>MSLTTFLFRNGALLDPDHPDLLQGFEILIEDGFIREVSDKPIKSSNAHVIDVKGKTIMPGLIDLHVHVVAIEFNLPRVATLPNVLVTLRAVPIMRAMLRRGFTTVRDAGGAGYPFKQAVESGLVEGPRLFVSGRALSQTGGHADPRARSDYMPPDSPCGCCVRVGALGRVADGVDEVRRAVREELQMGADQIKIMASGGVASPTDPVGVFGYSEDEIRAIVAEAQGRGTYVLAHAYTPAAIARAVRCGVRTIEHGNLIDDETARLVAEHGAYVVPTLVTYDALASEGEKYGLPPESIAKIADVHGAGLHSIEIMKRAGVKMGFGTDLLGEAQRLQSDEFRILAEVLSPAEVIASATIVSAEVLGMQDKLGRIVPGAHADVLVVDGNPLKSVDCLLGQGEHIPLVMKDGRLFV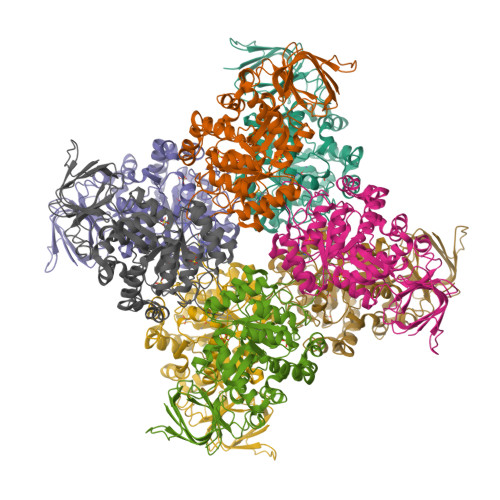NELEGHEGHHHHHH[8x]>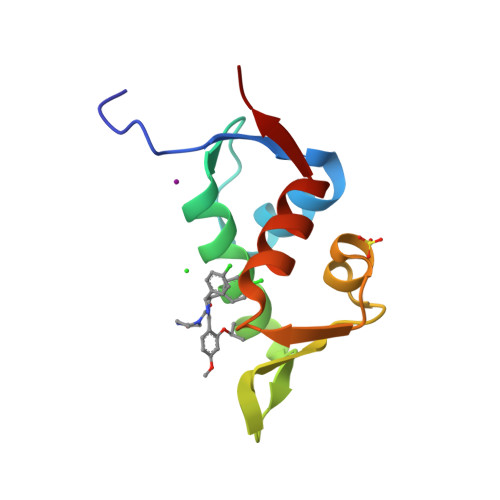PASEQETLVRPKPLLLKLLKSVGAQKDTYTMKEVLFYLGQYIMTKRLYDEKQQHIVYCSNDLLGDLFGVPSFSVKEHRKIYTMIYRNLVVVN[2x]>[2x]KKVVARVA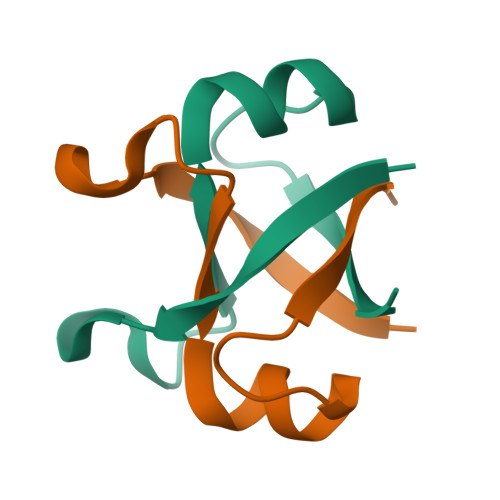EAYAEDVGKRVVRVDKYERAKVGVKVGDYVEVKKV>[8x]GSHMQSDSAVLQWANQAAIAAFTYNFVNYRDELQASSGFFTAEGWDQFLGALEQSNNLDAVKAKKLVVSAVATRAPIILQKGVLNGRYSWRVQMPILVTYQSASEFTQQNNVVTMLITRVS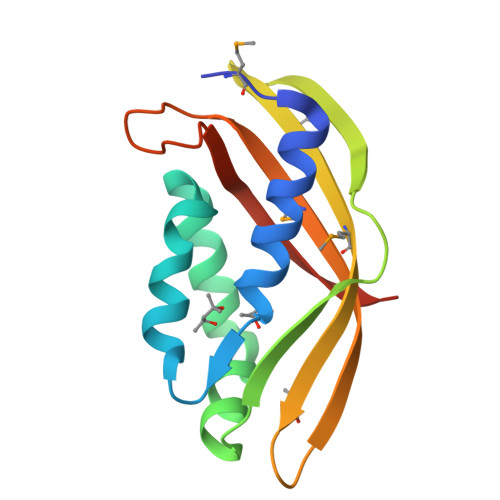TLNSPRGIGISQFVVGPASGGVS> GPLGSAKTRSIKSHEDLKQGEIVDGIVKNVNDKGIFVYLSRKVEAFVPVSKLSDSYLKEWK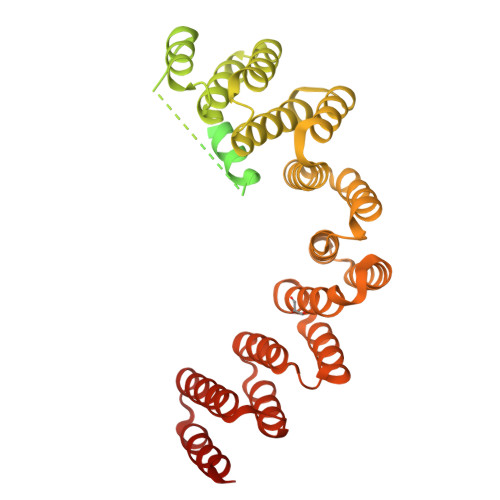KFYKPMQYVLGKVVTCDEDSRISLTLRESEINGDLKVLKTYSDIKAGDVFEGTIKSVTDFGVFVKLDNTVNVTGLAHITEIADKKPEDLSALFGVGDRVKAIVLKTNPEKKQISLSLKASHFSKEAELASTTTTTTTVDQLEKEDEDEVMADAGFNDSDSESDIGDQNTEVADRKPETSSDGLSLSAGFDWTASILDQAQEEEESDQDQEDFTENKKHKHKRRKENVVQDKTIDINTRAPESVADFERLLIGNPNSSVVWMNYMAFQLQLSEIEKARELAERALKTINFREEAEKLNIWIAMLNLENTFGTEETLEEVFSRACQYMDSYTIHTKLLGIYEISEKFDKAAELFKATAKKFGGEKVSIWVSWGDFLISHNEEQEARTILGNALKALPKRNHIEVVRKFAQLEFAKGDPERGRSLFEGLVADAPKRIDLWNVYVDQEVKAKDKKKVEDLFERIITKKITRKQAKFFFNKWLQFEESEGDEKTIEYVKAKATEYVASHESQKADE>[3x]AMADIGSDVASLRQQVEALQGQVQHLQAAFSQYKK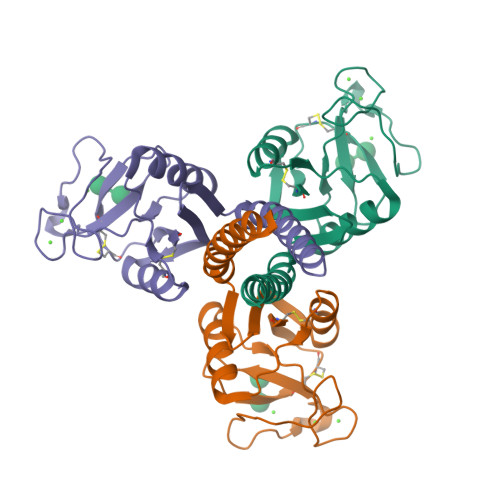VELFPNGQSVGEKIFKTAGFVKPFTEAQLLCTQAGGQLASPRSAAENAALQQLVVAKNEAAFLSMTDSKTEGKFTYPTGESLVYSNWAPGEPNDDGGSEDCVEIFTNGKWNDVACGEKRLVVCEF> MNSEYDYLFKLLLIGNSGVGKSCLLLRFSDDTYTNDYISTIGVDFKIKTVELDGKTVKLQIWDTAGQERFRTITSSYYRGSHGIIIVYDVTDQESFNGVKMWLQEIDRYATSTVLKLLVGNKCDLKDKRVVEYDVAKEFADANKMPFLETSALDSTNVEDAFLTMARQIKESMSQQNLNETTQKKEDKGNVNLKGQSLTNTGGGCC;> MGSSHHHHHHSQENLYFQGMVFSYEHYMNLLFHLDNSKETVPPEIAKRIISNAIAPVITVTSTPLFDKHIQETYKVDSLYMLLRFFGGCVSDRDQANEAKVGQHEHEVCDASDSTDSIPKNKNLEVPNLSKKGSRSRSNSLFQRDSTQSQYIRFTRPLGDLIETRDANDMLFNYHSLEVFLDNYLKLVAANTDEMVPHNLLKKSIYHSFFSLAISSTNNLSPYETFNHPILSLIALDISNGEVYEDARDLLVNFKNLNHNTENFPIFMNTNEMLPVFLLCYNDDSQEEFEKCQALAKKLKKQLFVESILLALWKDSFIYDENSVIQLHQPVMSSLEEILFFLQAPTQTTLSLALINSIYDMLDYLVYDLMIPFMKRKVSFWEETILQPRKSLFNGAKFFKKFMNKNPVNGNHQHNSLTRDSQGNEYFASSSSEFLMRKLADWSMMLSDFKTAYSTYESLMDDLDAFPKYLASCIEWCAVSLLMGAQSIVTVKMIKNDINPLIERALATYENCSRIQRGKGKESNSLDVTEPVRSYETRCMILASELFLSLSNTWTSTPYAIQYLETILDECKLGPCSQIMVWERLSDCYNLRVDPRIKHRVGAMKKDAKDTEDLRGEHKYSTDHFTDEDILSEGLTRRRKAAFFRLIAAKKWAEQKQWRQVSWCLKDIESTYSEIKFLHGNGLILSKLKNQLNLKDVDSAPRPSEKNLTRTSVSFIG;> MSSTHSNNVGHPQSSPQGPLTEQQRAQQQYQIFENSLPKVSQSVYQMLLNEMVPLAMGIERQISGDVISSDSNVTSENGNINNMIKRLKIEEHHTVDIIRSHNLIHELYKADEEEKEKVLARLRNIGFQIGLKLSELLIFSNNPNLKFKEMDLLLIMKFICRDVWKQIFGKQIDNLKTNHRGTFYLLDYDYRPIQSFSLEEDAKNEELKMIEPFLEIPVGIIRGVLSSLGYSSEEVICLASFIDRPTDRPKTAFPKGVSFHVQVTMPQ;>MVSTTQSRSLKAMGEEIWKNKTEKINTELFTLTYGSIVAQLCQDYERDFNKVNDHLYSMGYNIGCRLIEDFLARTALPRCENLVKTSEVLSKCAFKIFLNITPNITNWSHNKDTFSLILDENPLADFVELPMDAMKSLWYSNILCGVLKGSLEMVQLDCDVWFVSDILRGDSQTEIKVKLNRILKDEIPIGED[2x];> MGIYSFWIFDRHCNCIFDREWTLASNSASGTINSKQNEEDAKLLYGMIFSLRSITQKLSKGSVKNDIRSISTGKYRVHTYCTASGLWFVLLSDFKQQSYTQVLQYIYSHIYVKYVSNNLLSPYDFAENENEMRGQGTRKITNRNFISVLESFLAPMVNQ;> MAIETILVINKSGG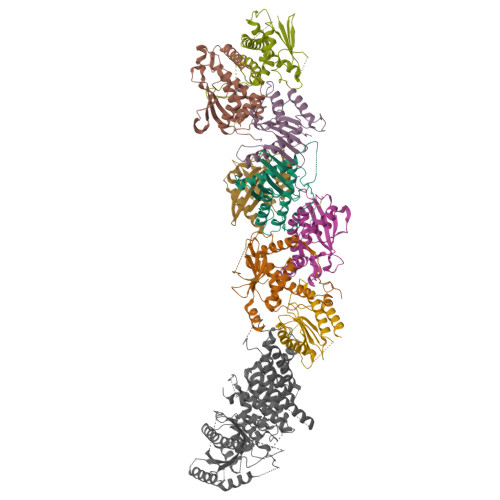LIYQRNFTNDEQKLNSNEYLILASTLHGVFAIASQLTPKALQLTQQTNIENTIPYIPYVGMSSNRSDTRNGGGNNNKHTNNEKLGSFKGDDFFKEPFTNWNKSGLRQLCTDQFTMFIYQTLTGLKFVAISSSVMPQRQPTIATTDKPDRPKSTSNLAIQIADNFLRKVYCLYSDYVMKDPSYSMEMPIRSNLFDEKVKKMVENLQ;> MSQRIIQPSASDQQFPGKSDGYEYTVGPKQAITSEASTTYIPSRIYSESLLFKRQEASLSAMAFLFQEMISQLHRTCKTAGDFETKLSDYGHNIGIRLLELLNFRASVSPSSLPRASAFLSQNESSSKLSNASNSPGMLANSSTATSASANERLQEKQTESLSNYITKMRRRDLKILDILQFIHGTLWSYLFNHVSDDLVKSSERDNEYMIVDNFPTLTQFIPGENVSCEYFVCGIIKGFLFNAGFPCGVTAHRMPQGGHSQRTVYLIQFDRQVLDREGLRFG;> MPQYFAIIGKKDNPVYEIEFTNAENPQGFPQDLKELNPFILHASLDIVEDLQWQINPTSQLNGNGGNGSNGGGGFLRSRAVNNTDNCYLGKVDHFYGLAITAYISYSGMKFVMIHGNSANSSVVIDDNNMRSFYQEVHELYVKTLMNPFYKITDPIRSPAFDSRVRTLARKHLSK>[2x]MLRMLSEAHGNVVLADDLPAKPVGVMKPGMVEIGAATHDRASRRSPTIRTTEALSRLTAVTATKIRRLAVVAPLGLACLCSGWPASSQVVIGPGDRPETGLQGQTTIEDVVSGRSKLPYHAGVRLVGRTDIWNRGGNLQLSWVDQCAYVSTFKQAGPITANSRSALFLREPAGVAVIDVRDPRAPKPVRLLRDRGSIDAVETMHAIAAPGRKVLVAGAYSGGIAGRGEEDAAWLSIYDASNCLNPKLQSEFKWPANIHMVTISPNGRRVYGTEVVPGLGSGKGGLHVLDISDMKRPRYLGRFGVTRP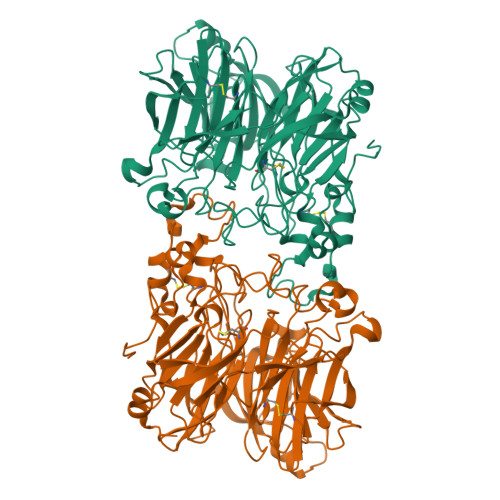NGLTAGFTPHEVSISHDERRIYAAVLASETGDVPVGASILASDGDVPVENGSVYILDNSDIVDGRSQPKMRLVGEAKQGGFHSVVPASINGVPHLVGAAELGACPGTWPRIINIADEKNPKIVGEFKLQMNIKENCDAIRFTPRKEDPYASFIPIPDITARLGAVGSHFNDVDDARNTRLGLFPFFAGGVRIVDLRDPTKPVEVGYYKPGANPDTPLSGNGLNWTGLNDQVTDGCMSHVRYVPESGHIWFACVTTGFHVVELNPDLRARLGFPTVKLEHHHHHH> NKTVLPIM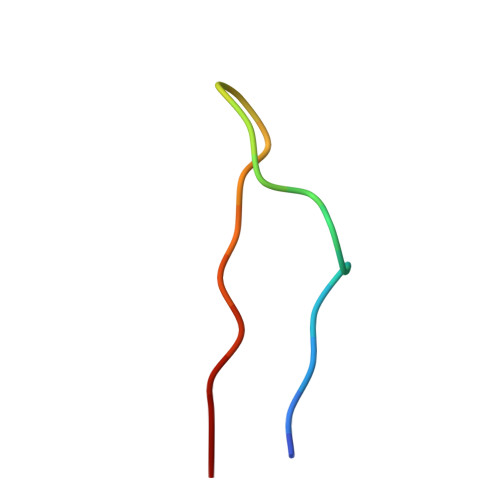SGFKFHSKPVIN We solved the 3-D structure of the Candida albicans CA3427 gene product, selected on the basis of its conservation among pathogenic fungi, and thus a potential target for new antifungal drugs. The structure of the protein unambiguously revealed a PBP fold, despite a low level of sequence similarity with previously known members of this family. CA3427 is an α/β protein with two domains organized into a C-clamp shape. The two domains delimit a large groove and are linked by a hinge region (residues 82–87 and 184–189).

Interestingly, two crystal forms were obtained which seem to correspond to a large conformational change induced by the binding of a small ligand at a specific site of the protein. The two crystal forms correspond to distinct conformations of the CA3427 protein with a root mean square deviation (RMSD) of 1.55 Å based on α-carbons superimposition of the overall structures. Most of the RMSD value results from a change in the relative position of the two domains rather than from local rearrangements (see Movie S1 for an animated view). When the PEG/acetates molecules are present in the structure, the E11-Oε2 forms a hydrogen bond with Y237-OH (distance 2.7 Å). Upon pointing outwards from the binding pocket, it clears the space needed to accommodate the ligand. In the second structure, the above distance becomes 4.5 Å and the E11 side chain now points towards the inner part of the cavity. The R112 side chain points towards the inside of the groove in the unliganded structure and outwards in the liganded one. Finally, in the closed conformation (i.e. without PEG/acetates molecules), D236-Oδ1 (Domain I) and K170-Nζ (Domain II) are linked by a salt bridge (distance 3 Å) that is disrupted in the presence of ligand (distance 4.8 Å), thus opening the “Venus flytrap”. The conformational change of the CA3427 protein upon ligand binding illustrates the venus fly trap motion already documented in other PBP structures.

> MAHHHHHHGHHHQLPTLKVAYIPEHFSTPLFFAQQQGYYKAHDLSIEFVKVPEGSGRLINLLNSNEVDIAIGLTEAFIADIAKGNENIHVLDTYVKSPLLWAVSTGSNRDDVTDAKQLKRIGVSRIGSGSYVMSFVLAHQLGVPSFDQFQVLSNFKNLRDSVNLKDGVEGSDAFMWEYFTSKKYYDNHEIKQIDQIYTPWSSWVVATSSDSLQAKSDVIKNFIDAVNQGIQYYNEHVDEAIEYISSNLDYSAEDAKEWTKTVEFNSRIGKTPLDWDTIVVKTKDTLKLAGVLAESDDVILKRLNSNVKKTNLQLDGDLEAA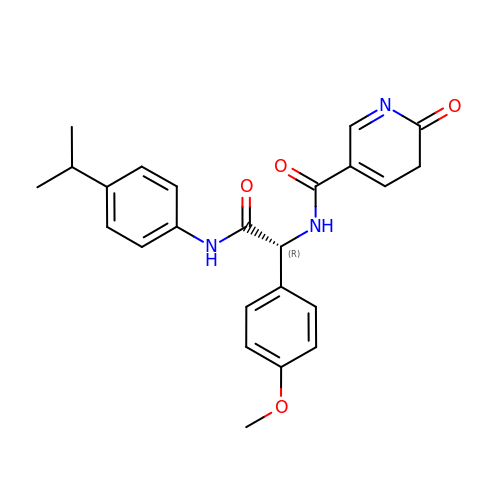~{N}-[(1~{R})-1-(4-methoxyphenyl)-2-oxidanylidene-2-[(4-propan-2-ylphenyl)amino]ethyl]-2-oxidanylidene-3~{H}-pyridine-5-carboxamide | C24 H25 N3 O4 | YAYNXABYSCGEEK-JOCHJYFZSA-N>[2x]MASSAQDGNNPLFSPYKMGKFNLSHRVVLAPMTRCRALNNIPQAALGEYYEQRATAGGFLITEGTMISPTSAGFPHVPGIFTKEQVREWKKIVDVVHAKGAVIFCQLWHVGRASHEVYQPAGAAPISSTEKPISNRWRILMPDGTHGIYPKP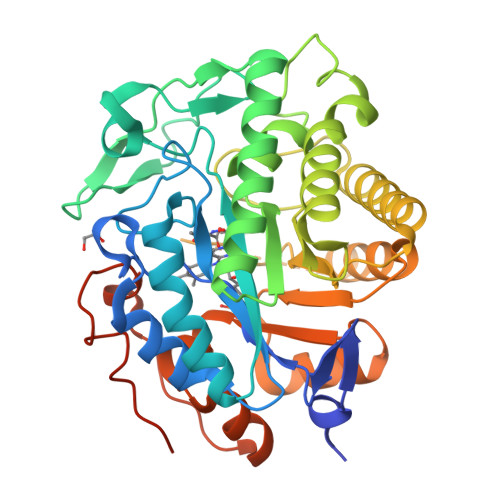RAIGTYEISQVVEDYRRSALNAIEAGFDGIEIHGAHGFLIDQFLKDGINDRTDEYGGSLANRCKFITQVVQAVVSAIGADRVGVRVSPAIDHLDAMDSNPLSLGLAVVERLNKIQLHSGSKLAYLHVTQPRYVAYGQTEAGRLGSEEEEARLMRTLRNAYQGTFICSGGYTRELGIEAVAQGDADLVSYGRLFISNPDLVMRIKLNAPLNKYNRKTFYTQDPVVGYTDYPFLQGNGSNGPLSRLLEHHHHHH>MSGKRIDEIESKLKHLEEFTTHLIKLMETMLELLKLVSDGKSDSEEYKELLEKAEEYLKQATEAAKKIGS[12x]

Here we use deep network hallucination to generate a wide range of symmetric protein homo-oligomers given only a specification of the number of protomers and the protomer length. Starting from only a choice of chain length L and oligomer valency N (2 for a dimer, 3 for a trimer, etc.), the method carries out a Monte Carlo search in sequence space starting from a random sequence. The loss function guiding the search is computed by inputting N copies of the sequence into the AlphaFold2 (AF2) network, and combining structure prediction confidence metrics (pLDDT; per-residue structural accuracy, and pTM; an estimate of the TM-score) with a measure of cyclic symmetry (the standard deviation of the distances between the center of mass of adjacent protomers within the predicted structure). To eliminate such over-fitting, we generated new sequences for the HAL backbones using the recently developed ProteinMPNN sequence design neural network (accompanying manuscript: Dauparas et al.).

To evaluate design accuracy we attempted crystallization of 19 designs and succeeded in solving crystal structures for seven (three C2s, two C3s and two C4s). All crystal structures had the correct oligomerization state and closely matched the design models (median Cα RMSD of 0.6 Å across all designs, with resolutions ranging from 1.8 to 3.4 Å). The side chain conformations in the crystal structures also closely match those of the design models. HALC3_104 is a homo-trimeric coiled-coil, with a central bundle of three helices, augmented by an outer-ring of three shorter helices that lie in the groove formed by adjacent protomer (the closest matching structure in the PDB has a TM-score of 0.88).> GSSHHHHHHSGDPASMNNHPEVKIKTILSLFLNINIDDFNMDANLADAYDMDXTELADLAKEIEKE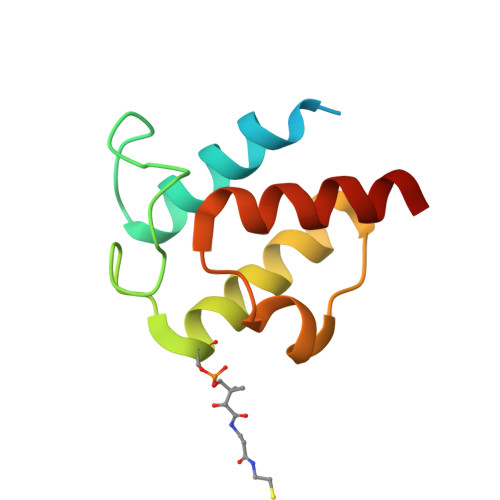FGISVTKSQFSHWETGRAVLDFVSSSLNDKN> GKDSCQG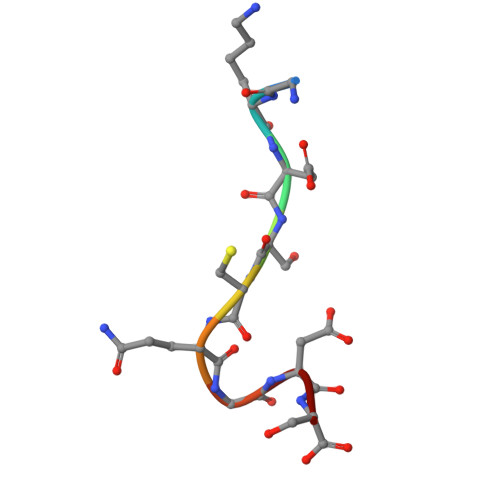DS Many proteins, including the EP300/CBP histone acetyltransferases (HATs), contain several targetable domains. EP300 and CBP broadly regulate the activity of other proteins through their protein acetyltransferase catalytic activity. These proteins contain several highly homologous domains, including KIX, bromodomains (BRDs) and HAT domains, through which they interact with, dock to, and acetylate target proteins, respectively. EP300/CBP are critical gene-regulatory targets in cancer, with existing high potency inhibitors of either the catalytic HAT domain or protein-binding bromodomain (BRD). Using crystallography, we identify the binding mechanism of the EP300/CBP-specific BRD inhibitor CCS1477 in complex with the EP300, CBP and BRD4 BRDs, and define components of the CCS1477 catalytic binding core that are required for compound activity.

Since recombinant CBP BRD was more robust in biochemical assays and crystallization studies, Kd values were determined for all compound-CBP interactions by MST, and co-crystal structures of the CBP BRD with five of the seven analogues were determined. Substitution of difluorophenyl with a less bulky phenyl (compound 5) resulted in a ~10-fold loss of binding activity, and the cocrystal revealed that R1173 is now hydrogen-bonded to the piperidinone oxygen but not quite close enough to the phenyl ring to establish a Pi-cation interaction. In contrast, milder changes to compound structure that retain the ability of compound to form Pi-cation as well as hydrogen-bonding interactions with the bromodomain result in only minor changes in IC50.

>KKIFKPEELRQALMPTLEALYRQDPESLPFRQPVDPQLLGIPDYFDIVKNPMDLSTIKRKLDTGQYQEPWQYVDDVWLMFNNAWLYNRKTSRVYKFCSKLAEVFEQEIDPVMQSLG[4x]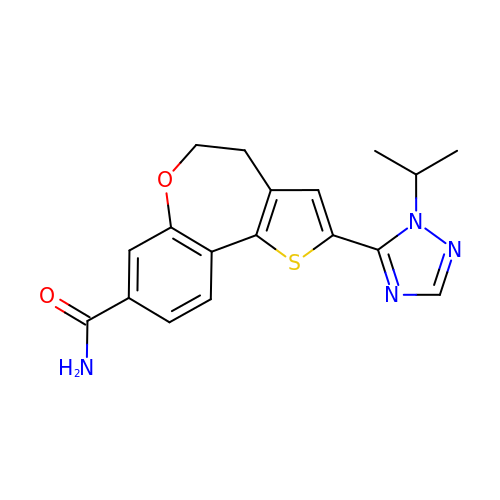2-[1-(propan-2-yl)-1H-1,2,4-triazol-5-yl]-4,5-dihydrothieno[3,2-d][1]benzoxepine-8-carboxamide | C18 H18 N4 O2 S | DJWGTNCIAUYYCQ-UHFFFAOYSA-N>MAKKKKKKSFNTTRPTDPPVYPVTVPFLGHIVQFGKNPLEFMQRCKRDLKSGVFTISIGGQRVTIVGDPHEHSRFFSPRNEILSPREVYTIMTPVFGEGVAYAAPYPRMREQLNFLAEELTIAKFQNFVPAIQHEVRKFMAENWKEDEGVINLLEDCGAMIINTACQCLFGEDLRKRLNARHFAQLLSKMESSLIPAAVFMPWLLRLPLPQSARCREARAELQKILGEIIVAREKEEASKDNNTSDLLGGLLKAVYRDGTRMSLHEVCGMIVAAMFAGQHTSTITTSWSMLHLMHPKNKKWLDKLHKEIDEFPAQLNYDNVMDEMPFAERCVRESIRRDPPLLMVMRMVKAEVKVGSYVVPKGDIIACSPLLSHHDEEAFPNPRLWDPERDEKVDGAFIGFGAGVHKCIGQKFALLQVKTILATAFREYDFQLLRDEVPDPDYHTMVVGPTLNQCLVKYTRKKKLPSHHHHHH[2x]

Trypansoma cruzi, the protozoan agent of Chagas Disease, is closely related to two other major global pathogens, Leishmania spp., responsible for leishmaniasis, and Trypansoma brucei, the causative agent of African Sleeping Sickness. Both T. cruzi and Leishmania parasites have an essential requirement for ergosterol, and are thus vulnerable to inhibitors of sterol 14α-demethylase (CYP51), which catalyzes the conversion of lanosterol to ergosterol. Here we report the crystal structures for the CYP51 target in T. cruzi (CYP51Tc) (resolutions 2.35 Å and 2.27 Å) and that of the closely related CYP51 ortholog from Trypanosoma brucei (CYP51Tb) (resolutions 2.7 Å and 2.6 Å), each bound to an anti-fungal triazole drug, either fluconazole or posaconazole. Nevertheless, CYP51Tc and CYP51Tb do share 83% sequence identity, a fact which has been crucial for successfully determining their crystal structures and makes it possible to extrapolate structural features learned from one enzyme toward the other.

Although largely a backbone trace at 3.2 Å resolution, this structure served as a search model for molecular replacement in determining the CYP51Tc–fluconazole structure at 2.35 Å, which was used as a search model against the 2.27 Å CYP51Tc–fluconazole data to reveal an alternative conformation of fluconazole bound in the active site. The two CYP51Tc–fluconazole structures reported here superimpose with r.m.s.d of 0.68 Å, revealing some conformational differences in the F-helix and the BC-loop, which may account for the distinct fluconazole binding modes and result in re-packing of protein molecules in the crystal lattice. As expected, fluconazole is bound in the active site by coordination to the heme iron via the aromatic nitrogen atom of a triazole ring and by multiple van der Waals and aromatic stacking interactions. The 2,4-difluorophenyl moiety is enclosed in the pocket formed by the heme macrocycle, the aromatic side chains of Y103, F110, Y116 (BC-loop) and F290 (I-helix), and aliphatic side chains M106, A287 and A291. Although fluconazole occupies the same pocket in both CYP51Tc structures, it adopts two conformations that differ by the 180° flipping of the 2,4-difluorophenyl moiety. A 2.6 Å H-bonding contact between the 2-fluoro substituent and the hydroxyl group of Y103 may help to stabilize orientation 2, which appears to be less sterically favorable than orientation. In orientation 1, the H-bond between the 2-fluoro substituent and Y103 is broken due to the 3.5 Å reorientation of Y103 toward M360 resulting in the 2.7 Å H-bond to its amide nitrogen and in the flipping of the 2,4-difluorophenyl ring into a sterically more favorable orientation with the fluorinated edge facing away from the heme macrocycle. Perhaps both ring conformations co-exist in the CYP51Tc-fluconazole complex, possibly correlated with the conformation of the BC-loop which affects H-bonding pattern of Y103.>[4x]MERPQPDSMPQDLSEALKEATKEVHTQAENAEFMRNFQKGQVTRDGFKLVMASLYHIYVALEEEIERNKESPVFAPVY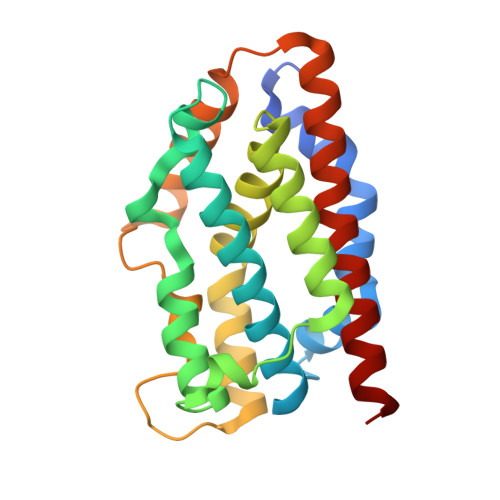FPEELHRKAALEQDLAFWYGPRWQEVIPYTPAMQRYVKRLHEVGRTEPELLVAHAYTRYLGDLSGGQVLKKIAQKALDLPSSGEGLAFFTFPNIASATKFKQLYRSRMNSLEMTPAVRQRVIEEAKTAFLLNIQLFEELQELLTHD>MAHAPGTDQMFYVGTMDGWYLDTKLNSVAIGAHWSCFIVLTITTFYLGYESWTSRGPSKRTSFYAGYQEEQNLALFVNFFAMLSYFGKIVADTLGHNFGDVGPFIIGFGNYRYADYMLTCPMLVYDLLYQLRAPYRVSC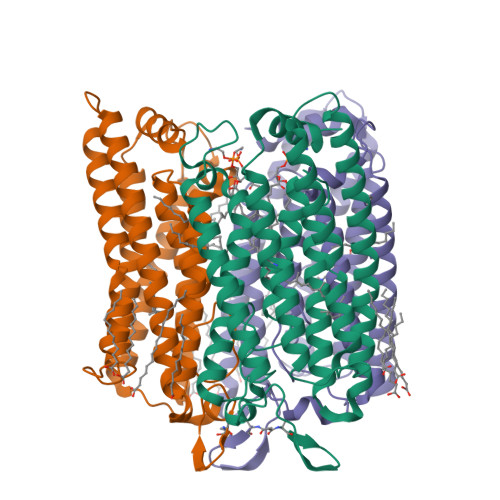SAIIFAILMSGVLAEFYAEGDPRLRNGAYAWYGFGCFWFIFAYSIVMSIVAKQYSRLAQLAQDTGAEHSLHVLKFAVFTFSMLWILFPLVWAICPRGFGWIDDNWTEVAHCVCDIVAKSCYGFALARFRKTYDEELFRLLEQLGHDEDEFQKLELDMRLSSNGERLRRLSLNSLEVLFQ[3x]alpha-D-allopyranose | 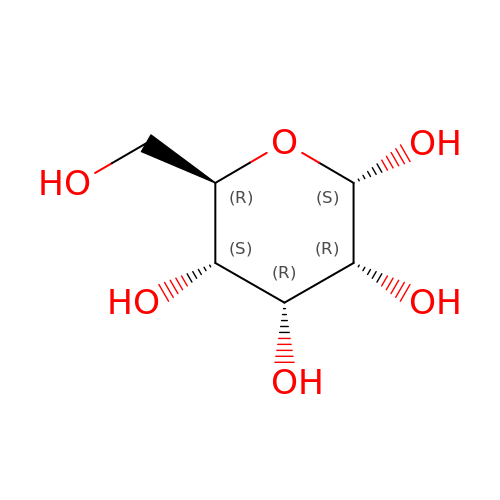C6 H12 O6 | WQZGKKKJIJFFOK-UKFBFLRUSA-N> GLGDELEEVIVEKTKQTVASISSGPKHTQKVPILTANETGATMPVLPSDSIETRTTYMHFNGSETDVECFLGRAACVHVTEIQNKDATGIDNHREAKLFNDWKINLSSLVQLRKKLELFTYVRFDSEYTILATASQPDSANYSSNLVVQAMYVPPGAPNPKEWDDYTWQSASNPSVFFKVGDTSRFSVPYVGLASAYNCFYDGYSHDDAETQYGITVLSHMGSMAFRIVNEHDEHKTLVKIRVYH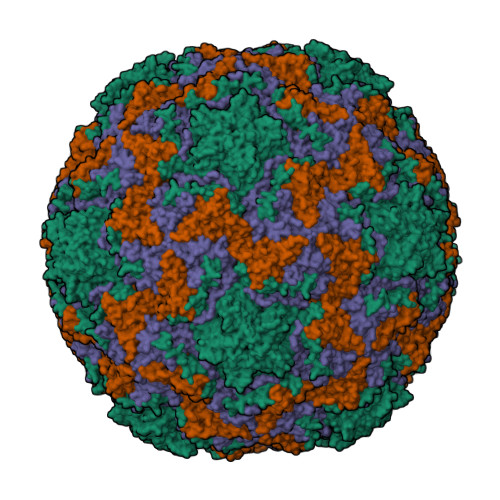RAKHVEAWIPRAPRALPYTSIGRTNYPKNTEPVIKKRKGDIKSY;> SPNVEACGYSDRVQQITLGNSTITTQEAANAVVCYAEWPEYLPDVDASDVNKTSKPDTSVCRFYTLDSKTWTTGSKGWCWKLPDALKDMGVFGQNMFFHSLGRSGYTVHVQCNATKFHSGCLLVVVIPEHQLASHEGGNVSVKYTFTHPGERGIDLSSANEVGGPVKDVLYNMNGTLLGNLLIFPHQFINLRTNNTATIVIPYINSVPIDSMTRHNNVSLMVIPIAPLTVPTGATPSLPITVTIAPMCTEFSGIRSKSIVPQ;> GLPTTTLPGSGQFLTTDDRQSPSALPNYEPTPRIHIPGKVHNLLEIIQVDTLIPMNNTHTKDEVNSYLIPLNANRQNEQVFGTNLFIGDGVFKTTLLGEIVQYYTHWSGSLRFSLMYTGPALSSAKLILAYTPPGARGPQDRREAMLGTHVVWDIGLQSTIVMTIPWTSGVQFRYTDPDTYTSAGFLSCWYQTSLILPPETTGQVYLLSFISACPDFKLRLMKDTQTISQTVALTE;> GAQVSTQKSGSHENQNILTNGSNQTFTVINYYKDAASTSSAGQSLSMDPSKFTEPVKDLMLKGAPALN>[2x]AWKVSVDQDTCIGDAICASLCPDVFEMNDEGKAQPKVE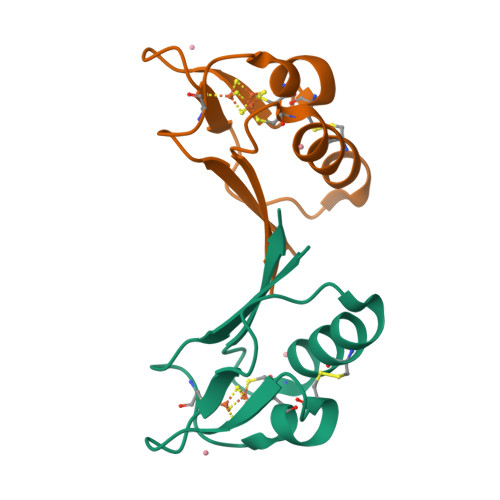VIEDEELYNCAKEAMEACPVSAITIEEA>[2x]SNAVGQFANFVDLLQYRAKLQARKTVFSFLADGEAESAALTYGELDQKAQAIAAFLQANQAQGQRALLLYPPGLEFIGAFLGCLYAGVVAVPAYPPRPNKSFDRLHSIIQDAQAKFALTTTELKDKIADRLEALEGTDFHCLATDQVELISGKNWQKPNISGTDL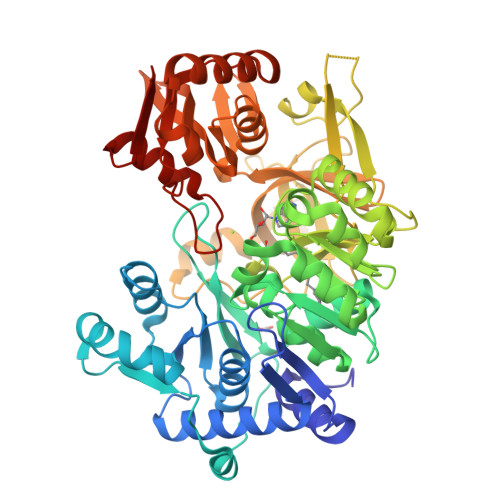AFLQYTSGSTGDPKGVMVSHHNLIHNSGLINQGFQDTEASMGVSWLPPYHDMGLIGGILQPIYVGATQILMPPVAFLQRPFRWLKAINDYRVSTSGAPNFAYDLCASQITPEQIRELDLSCWRLAFSGAEPIRAVTLENFAKTFATAGFQKSAFYPCYGMAETTLIVSGGNGAAQLPQEIIVSKQGIEANQVRPAQGTETTVTLVGSGEVIGDQIVKIVDPQALTECTVGEIGEVWVKGESVAQGYWQKPDLTQQQFQGNVGAETGFLRTGDLGFLQGGELYITGRLKDLLIIRGRNHYPQDIELTVEVAHPALRQGAGAAVSVDVNGEEQLVIVQEVERKYARKLNVAAVAQAIRGAIAAEHQLQPQAICFIKPGSIPKTSSGKIRRHACKAGFLDGSLAVVGEWQ In this study, we have determined the crystal structures of bcPadR1 and bcPadR2, which are the products of gene loci BC4206 and BCE3449 of B. cereus strains ATCC 14579 and ATCC 10987, respectively. The bcPadR1 and bcPadR2 subunits contain a typical wHTH DNA-binding domain, consisting of helices α1, α2, the DNA recognition helix α3 and strands β1 and β2 (together forming the wing), and a dimerization domain, including the C-terminal helix α4. Unlike LmrR, but like the other PadR-s2 proteins with known structure, the bcPadR1 and bcPadR2 dimers have a completely closed dimer interface. The closed dimer conformation and inaccessibility of the conserved tryptophan residues of the bcPadR proteins are incompatible with a drug-binding mechanism as observed in LmrR.

Here we report the crystal structure of the BC4206 gene product from B. cereus strain ATCC 14579, a subfamily-2 PadR-like protein which we named bcPadR1. The gene encoding bcPadR1 (locus BC4206 in B. cereus ATCC 14579) is located immediately downstream from BC4207, encoding a putative membrane protein of unknown function. Transcriptome analysis revealed that BC4206 and BC4207 are co-upregulated in response to enterocin AS-48, indicating that these genes indeed form a bicistronic transcriptional unit. Overexpression results in an increased sensitivity against AS-48 (MIC value of 1.0 µg/ml compared to a MIC value of 2.5 µg/ml for the wild-type strain, p-value<0.005, >6 cultures as determined with Student's t-test) suggesting that bcPadR1 acts as a repressor of the BC4206-BC4207 transcriptional unit, when AS-48 is not present in the medium. Electrophoretic mobility shift assays further reveal that purified bcPadR1 specifically binds to the intergenic region between BC4205 and the BC4206-BC4207 operon. In vitro DNA binding of bcPadR1 was not affected by the addition of AS-48 suggesting an indirect sensing of AS-48 in the medium, although we cannot exclude the possibility that slightly altered in vitro conditions (e.g. different binding buffer) are needed to observe any effect of AS-48 addition on DNA binding. BcPadR1 was crystallized in space group P41212, with one protein molecule per asymmetric unit and a solvent content of 71%. As these interactions are crucial for the strong DNA binding affinity of RTP, it is likely that the conserved residues in bcPadR1 and bcPadR2 have a similar DNA binding role. This is corroborated by the observation of a bound sulfate anion in the bcPadR1 structure, which forms interactions with the highly conserved residues Gly25, Tyr26, Glu42 Arg71, and Lys72, likely mimicking the interactions with a phosphate moiety of the DNA backbone. The bcPadR1 dimer can be superimposed to the DNA-bound complexes of RTP and BlaI with RMSD values of 3.5 Å (for 176 common Cα atoms divided equally between both subunits) and 4.1 Å (for 153 common Cα atoms), respectively.

> MHSQMLKGVLEGCILYIISQEEVYGYELSTKLNKHGFTFVSEGSIYPLLLRMQKEKLIEGTLKASSLGPKRKYYHITDKGLEQLEEFKQSWGMVSTTVNNLLQGESRWSHPQFEK>GHMNAQARFSQNLLDQGSHPTSEKLLSVLRPASGHVADALGITEGENVIHLRTLRRVNGVALCLIDHYFADLTLWPTLQRFDSGSLHDFLREQTGIALRRSQTRISARRAQAKECQRLEIPNMSPLLCVRTLNH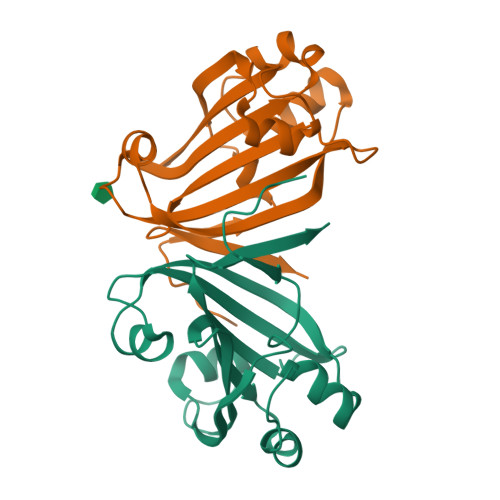RDGESSPAEYSVSLTRADMIEFTMEH[2x]> MAHHHHHHSSGLEVLFQGPGPLLVPRVKVAEDGSIILDEESLTVEVLRTKGPCVVEENDPIFERGSTTTYSSFRKNYYSKPWSNKETDMFFLAISMVGTDFSMIGQLFPHRARIEIKNKFKREEKTNGWRIDKAFQEKRPFDF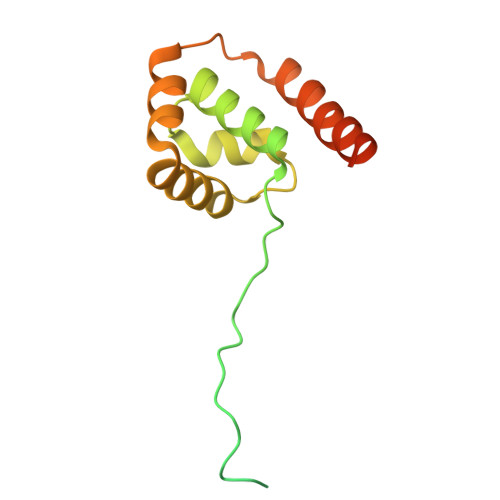DFFAHLLQKVLAEEEKRKQKSVKNHSLKEKKS> CDKSTDDTSKVTYFVTLEREGDEKIVLEKGQPFVEPGYYAEMN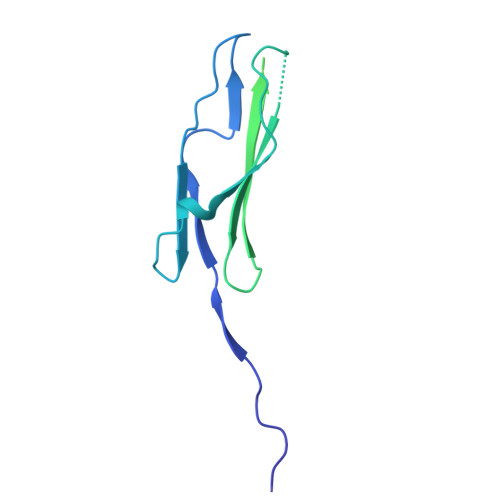GEDITESVQIKGSVDVNTPGIYNLVYAAYNEDGFAKTFTRTVYVADNTASPLKSGIYTVAEGSKRTAPSVVAFSGYEIVIFQMEPGIFYISDFLGGWYDQRAGYGPDYAMVGKFELNDDNTITPLESYVAGWGDSMDQMTNTLLDPATGTLKWTVAYAGQLSFDIIVKQ> MAKALIVYGSTTGNTEYTAETIARELADAGYEVDSRDAASVEAGGLFEGFDLVLLGCSTWGDDCIELQDDFIPLFDSLEETGAQGRKVACFGCGDSSYEYFCGA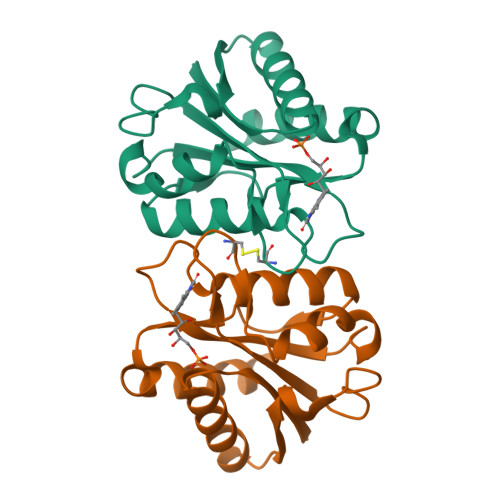VDAIEEKLKNLGAEIVQDGLRIDGDPRAARDDIVGWAHDVRGAI Here, we identify an alternative approach to sulfoquinovoside hydrolysis that is adopted by these organisms and discover a family of SQases belonging to a new glycoside hydrolase family (GH188). These new SQases operate through an oxidoreductive mechanism that results in net hydrolysis and involves a catalytic NAD+ cofactor. The SqgA proteins adopt a two-domain fold with an N-terminal dinucleotide binding Rossmann domain and a C-terminal α/β dimerization domain. The structures reveal homodimers, consistent with molar mass analysis using size-exclusion chromatography-multiangle laser light scattering in solution.

FlSqgA from Flavobacterium sp. strain K172 was selected for further study. Further analysis revealed that the small increase in product formation observed in the presence of Mn2+ was a result of improved enzyme stability; thus, Mn2+ was included in subsequent kinetic studies. These data show that FlSqgA is a metal-independent NAD+-dependent SQase. No activity was observed against 4-nitrophenyl α- and β-glucosides or 4-nitrophenyl β-glucuronic acid, showing that FlSqgA is specific for SQ glycosides. Another feature of NAD+-dependent glycosidases is the ability of many members to act on both α- and β-linked glycosides. Both 4-nitrophenyl α- and β-sulfoquinovosides (α-PNPSQ and β-PNPSQ) were substrates with the following Michaelis–Menten kinetic parameters: α-PNPSQ, kcat = 0.025 ± 0.002 s–1, KM = 2.9 ± 0.8 mM, and kcat/KM = 0.012 ± 0.001 mM–1 s–1; β-PNPSQ, kcat = 0.014 ± 0.002 s–1, KM = 1.7 ± 0.6 mM, and kcat/KM = 0.008 ± 0.001 mM–1 s–1. Soaking and cocrystallization experiments provided structures of the ArSqgA·NAD+·SQ and FlSqgA·NAD+·SQ complexes, which diffracted to 2.4 and 2.3 Å, respectively. Both ternary complexes were essentially identical, with respect to the active site interactions. Three-dimensional X-ray structures of complexes with SQ and NAD+ provide insight into the catalytic mechanism, which involves transient oxidation at C3.

>[4x]MGSSHHHHHHSSGMSLPSGETAQTIRYGLIGAGHMAREHVRNLALIPGSLITAVADPTPSSLEETAREIGYDVQTFSAHKDLLASGLVDALVIASPNDTHLEILKDIFASGTNLPVLVEKPVCTSAEQADELEELAATYTAPVWVAMEYRYMPPVQEIIQAAHSGKLGNIHMLSIVEHRFPFLHKVDAWNRFAERTGGTLVEKCCHFFDLMRLILQDEPTRIYASGGHDVNHMDEVYDGLISDMVDNAYVIVDFKGGRRAMLELSMFAEGSKFQERISIVGDAAKIETLIPVAANHWIEGDETEATVEFSPRSPLGPEKHEVPVDEAVLAAGAHHGSTYYEHLGYRKAILGEGPVDVTVADGLQSVRMGLAAEQSIIEGRAVELHAPSVAVQK>MTDAATAPTSIDLRAEYEGSGAKEVLEELDRELIGLKPVKDRIRETAALLLVERARQKLGLAHETPTLHMSFTGNPGTGKTTVALKMAG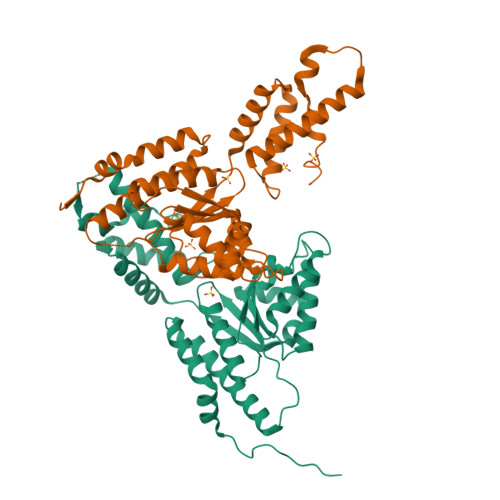LLHRLGYVRKGHLVSVTRDDLVGQYIGHTAPKTKEVLKRAMGGVLFIDEAYYLYRPDNERDYGQEAIEILLQVMENNRDDLVVILAGYADRMENFFQSNPGFRSRIAHHIEFPDYSDEELFEIAGHMLDDQNYQMTPEAETALRAYIGLRRNQPHFANARSIRNALDRARLRQANRLFTASSGPLDARALSTIAEEDIRASRVFKGGLDSERRAAEALAR[2x]BA0330 and BA0331 are the only lipoproteins among the 11 known or putative polysaccharide deacetylases of Bacillus anthracis. BA0330 and BA0331 from B. anthracis are predicted as lipoproteins and putative PDAs and share 55% sequence identity. BA0330 and BA0331 interact with peptidoglycan, and BA0330 is important for the adaptation of the bacterium to grow in the presence of a high concentration of salt, whereas BA0331 contributes to the maintenance of a uniform cell shape. Our data suggest that BA0330 and BA0331 have a structural role in stabilizing the cell wall of B. anthracis.

We next determined the crystal structure of BA0330 at 1.48 Å, which revealed two domains. In addition to the CE4-type esterase domain, there is an N-terminal fibronectin type 3 (Fn3)-like domain (residues 45–141) consisting of a two-layered (4 + 3) β-sandwich. Apart from the closely related BC0361 and BA0331 no other CE4 esterase studied so far has an Fn3-like domain. Part of the expressed protein (residues 24–44 of the N terminus) could not be determined in the electron density maps, and therefore the corresponding region was not built in the model. The CE4 domain resembles that of other deacetylases, containing a well formed groove with the zinc atom located at the bottom. The electron density at the binding site was attributed to the zinc ion, which is coordinated in a trigonal bipyramidal manner by two histidines, one aspartic acid, a water molecule, and an acetate molecule, probably present as a contaminant to the PEG solutions used in the crystallization buffer. One of its oxygens interacts with the invariant Asp205, which is tethered with Arg343 (present only in Fn3 domain-containing deacetylases), whose guanidinium group overlaps spatially with the corresponding group of SpPgdA-Arg364. The other acetate oxygen accepts a hydrogen bond at 2.9 Å from the hydroxyl group of the modified proline (Pro302), which was modeled as an α-hydroxy-l-proline located at a distance of 3.6 Å from the metal ion. Interestingly, Arg345 is found in place of a conserved aspartic acid that is believed to be responsible for tuning the pKa value of the catalytic histidine (His150). The structure of BA0330 reveals a differentiation of the catalytic machinery of PDAs and could explain the apparent lack of activity of this protein.

>[2x]MRKYAAIALCTSAILAGCNTSNVSQEPNKERKVQETKKQAETVQEQGKISYNPITHESTNTTIHMTDIKDTLTEVQYKIWRTADGKETAKSLSSKEKEKQFSLPFDTKEFEGKRGEFQIEAIGIKEDGKTIPLTKSAITFEQKVPVLMYHAIDDYHGQGIKDLFVSPANFEAQMKYLKDNGYTLLTFERWGDINKVNKPIFVTFDDGMKNNMNAFHVLQKLKDDTFKPVATEYMIVNNVDAEGSLSTSDIKEMVDSGIFSMQSHTATHADLPKITNYEEELKESKEKLEKITGKPVIAVAYXFGHVDDKVVAETKKYYQFATTTKPGKFITKGEPDELLKMKRVRIHHTTTVEQFASSIK> MGHHHHHHGSGSNRLDGKVAIITGGTLGIGLAIATKFVEEGAKVMITGRHSDVGEKAAKSVGTPDQIQFFQHDSSDEDGWTKLFDATEKAFGPVSTLVNNAGIAVNKSVEETTTAEWRKLLAVNLDGVFF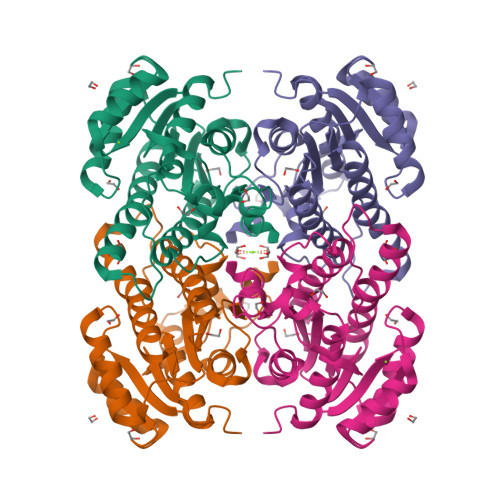GTRLGIHRMKNKGLGASIINMSSIEGFVGDPSLGAYNASKGAVRIMSKSAALDCALKDYDVRVNTVHPGYIKTPLVDDLPGAEEAMSQRTKTPMGHIGEPNDIAYICVYLASNESKFATGSEFVVDGGYTAQ Although no X-ray crystal structure of human GBA2 is available, structures have been solved for Thermoanaerobacterium xylanolyticumTxGH116 β-glucosidase, which shares 37% amino acid sequence identity with human GBA2.8 Instead of hydrolyzing glucosylceramide like GBA2, TxGH116 exhibits high activity toward 4-nitrophenyl β-D-glucopyranoside (4NPGlc), and β-1,3- and β-1,4-linked glucooligosaccharides. The TxGH116 structure contains an N-terminal domain, formed by a two-sheet β-sandwich, tightly associated with a C-terminal (α/α)6 solenoid domain that contains the catalytic nucleophile, E441, and general acid/base, D593, residues, which were verified by chemical rescue of alanine mutants. GH116 enzymes are retaining GHs, as shown for Saccharolobus solfataricus SSO1353 β-glucosidase/β-xylosidase, human GBA2, and TxGH116.6,8,12 In the retaining mechanism, catalysis involves two carboxylic acid/carboxylate side chains with one serving as an acid/base and the other as a nucleophile. Here, we report the structures of Thermoanaerobacterium xylanolyticum β-glucosidase (TxGH116) D593N acid/base mutant in complexes with cellobiose and laminaribiose and its catalytic mechanism.

The D593A and D593N unliganded enzymes and D593N complexes crystallized in the space group P21212, isomorphous, with wild-type TxGH116 crystals, whereas the crystals of TxGH116 D593A in complex with cellobiose and laminaribiose crystallized in the P212121 space group and had 2 molecules in one asymmetric unit. Comparison with the structure of the complex of D593A with cellobiose shows that in D593A the loop containing the catalytic acid/base, residues 585–596, is shifted and T591 does not interact with the nonreducing glucose residue while Y62 makes an addition interaction with the reducing end glucose residue. Nonetheless, the cellobiose is in a very similar position, suggesting no unusual effect on the substrate position is induced by hydrogen bonding to N593 in the D593N mutant. In each structure, the glucosyl residues at subsites –1 and +1 bind to the acid/base mutants in a relaxed 4C1 chair conformation.

>[2x]AMALTGCSEKININEDKISHKIDIPDSAWTIGIGEKFKNAGHPNVKYPMIDDSYVQGAPLGGFGAGTIGRTYNGGFSRWHLEIGKNKYTTVYANQFSVFQKVEGNKDGVAQVLYAGEPENGYLSSWKWDYPKESGMYYALYPNSWYTYTNKDLPVQLAVKQFSPIIPYNYKETSYPVAVFKWTAYNPTNKNVDVSIMFTWQNMIGFFGKQVNVNSGNFNKIIKDKSKDSEIVAAVMGNISNDNEEWNGEYSIGVKKVPGVDISYKAKFVTTGDGSDLWHEFSKNGILDNKDDETPTKQDGIGSAIAVNFKLQPGQTIEVPFALSWDLPIMKFGGGDKWYKMYTKYFGKNGKNSFAILKEALNNYQKWEKMIDDWQKPILSNKSKPDWYKTALFNELYYLADGGTAWENGKVGEKDKRTNNMFGLLECFDYNYYETLDVRFYGSFPLVMLWPDIEKQVMRQFADTINVQDSSEFKVGSNGAMAVKKVQGMIPHDLGSSYALPWIKINAYDWQNPNIWKDLNSKYVLLVYRDYVLTGKTDKEFLKYTWKSVKTALDKLKEMDKDNDGIPDNEGIPDQTYATWSMKGTSAYCGSLWLAALKAAQEIGKVLKDNEAYIKYNEWYKIAQQNFEKELWNGEYYNFDTESDHKDSIMADQLAGQWYADILRLGDILPKDHVQKALKKIYEFNVMKFENGKMGAVNGMRPDGIVDESDIQAQEVWTGVTYALASFMKYRGMTEEAYNTAYGVYKMTYDKSGKGYWFRTPEAWTKDGNYRASMYMRPLSIWSMEVNYNEVLEHHHHHH Central to this process is the ATP-sensitive potassium (KATP) channel assembled from four pore-forming Kir6.2 subunits (encoded by KCNJ11) and four regulatory SUR1 subunits (encoded by ABCC8). KATP channels are gated by intracellular ATP and ADP, the concentrations of which change following glucose metabolism. This enables KATP channels to couple blood glucose levels with β-cell membrane potential to control insulin secretion. SUR1, a member of the ABC protein family, consists of a canonical ABC core structure of two 6-TM helix TM domains (TMD), TMD1 and TMD2, and two cytoplasmic nucleotide binding domains (NBDs), NBD1 and NBD2; in addition, it contains an N-terminal TM domain TMD0 which is connected to the ABC core via a cytoplasmic linker, L0.

To directly visualize how Aekatperone interacts with the channel we determined the cryoEM structure of KATP channels in the presence of 50 μM Aekatperone, using our published cryoEM sample preparation, imaging, and data processing workflow with specific modifications. 3D reconstruction of cryoEM particles of channels incubated with Aekatperone yielded a map with an overall resolution of 4.1 Å. A model built from the map shows a closed Kir6.2 channel pore with a pore radius of ~0.75 Å at the helical bundle crossing residue F168 and an inward-facing SUR1 with NBDs separated, resembling other inhibitor-bound KATP channel structures reported to date. A clear nonprotein density consistent with the size of Aekatperone (MW: 399.52 g/mol) was observed in a TM pocket above NBD1 in the ABC core of SUR1. Moreover, as in the structures of KATP bound to GBC, RPG, or CBZ, we observed clear cryoEM density corresponding to the Kir6.2 distal N-terminal peptide domain (KNtp) in between the two TM bundles of the SUR1-ABC core, with the very N-terminus of Kir6.2 contacting the bound Aekatperone. Stabilization of the KNtp-SUR1 interface promotes channel assembly, at the same time, it prevents Kir6.2 cytoplasmic domain from rotating to an open conformation, which explains the dual chaperone and inhibitor activity of Aekatperone. Aekatperone comprises a cyclohexane ring, a pyrazole, a sulfonamide moiety, a benzene ring, and an imidazole group. The preferred binding conformation, which accounted for the physical chemical properties of the compound and its surrounding interacting protein residues as well as fit to the cryoEM density, is shown in Figure 5B and C. In this structural model, the cyclohexyl moiety of Aekatperone is aligned with S1238 on the cytoplasmic end of the binding pocket, and the imidazole group is oriented toward the extracellular end of the binding pocket, interacting with the distal part of KNtp. The pyrazole moiety has its two nitrogen atoms coordinated by T1242 and N1245, while the sulfonyl moiety is oriented toward R1246 and R1300, each interacts with one of the two oxygens of the sulfonyl group.

>[4x]MLSRKGIIPEEYVLTRLAEDPTEPRYRTRERRARFVSKKGNCNVAHKNIREQGRFLQDVFTTLVDLKWPHTLLIFTMSFLCSWLLFAMVWWLIAFAHGDLAPGEGTNVPCVTSIHSFSSAFLFSIEVQVTIGFGGRMVTEECPLAILILIVQNIVGLMINAIMLGCIFMKTAQAHRRAETLIFSKHAVITLRHGRLCFMLRVGDLRKSMIISATIHMQVVRKTTSPEGEVVPLHQVDIPMENGVGGNSIFLVAPLIIYHVIDSNSPLYDLAPSDLHHHQDLEIIVILEGVVETTGITTQARTSYLADEILWGQRFVPIVAEEDGRYSVDYSKFGNTVKVPTPLCTARQLDEDRSLLDALTLASSRGPLRKRSVAVAKAKPKFSISPDSLS;> MPLAFCGTENHSAAYRVDQGVLNNGCFVDALNVVPHVFLLFITFPILFIGWGSQSSKVHIHHSTWLHFPGHNLRWILTFILLFVLVCEIAEGILSDGVTESRHLHLYMPAGMAFMAAITSVVYYHNIETSNFPKLLIALLIYWTLAFITKTIKFVKFYDHAIGFSQLRFCLTGLLVILYGMLLLVEVNVIRVRRYIFFKTPREVKPPEDLQDLGVRFLQPFVNLLSKGTYWWMNAFIKTAHKKPIDLRAIGKLPIAMRALTNYQRLCVAFDAQARKDTQSPQGARAIWRALCHAFGRRLILSSTFRILADLLGFAGPLCIFGIVDHLGKENHVFQPKTQFLGVYFVSSQEFLGNAYVLAVLLFLALLLQRTFLQASYYVAIETGINLRGAIQTKIYNKIMHLSTSNLSMGEMTAGQICNLVAIDTNQLMWFFFLCPNLWAMPVQIIVGVILLYYILGVSALIGAAVIILLAPVQYFVATKLSQAQRSTLEHSNERLKQTNEMLRGMKLLKLYAWESIFCSRVEVTRRKEMTSLRAFAVYTSISIFMNTAIPIAAVLITFVGHVSFFKESDLSPSVAFASLSLFHILVTPLFLLSSVVRSTVKALVSVKKLSEFLSSAEIREEQCAPREPAPQGQAGKYQAVPLKVVNRKRPAREEVRDLLGPLQRLAPSMDGDADNFCVQIIGGFFTWTPDGIPTLSNITIRIPRGQLTMIVGQVGCGKSSLLLATLGEMQKVSGAVFWNSNLPDSEGEDPSSPERETAAGSDIRSRGPVAYASQKPWLLNATVEENITFESPFNKQRYKMVIEACSLQPDIDILPHGDQTQIGERGINLSGGQRQRISVARALYQQTNVVFLDDPFSALDVHLSDHLMQAGILELLRDDKRTVVLVTHKLQYLPHADWIIAMKDGTIQREGTLKDFQRSECQLFEHWKTLMNRQDQELEKETVMERKASEPSQGLPRAMSSRDGLLLDEEEEEEEAAESEEDDNLSSVLHQRAKIPWRACTKYLSSAGILLLSLLVFSQLLKHMVLVAIDYWLAKWTDSALVLSPAARNCSLSQECDLDQSVYAMVFTLLCSLGIVLCLVTSVTVEWTGLKVAKRLHRSLLNRIILAPMRFFETTPLGSILNRFSSDCNTIDQHIPSTLECLSRSTLLCVSALTVISYVTPVFLVALLPLAVVCYFIQKYFRVASRDLQQLDDTTQLPLLSHFAETVEGLTTIRAFRYEARFQQKLLEYTDSNNIASLFLTAANRWLEVRMEYIGACVVLIAAATSISNSLHRELSAGLVGLGLTYALMVSNYLNWMVRNLADMEIQLGAVKRIHALLKTEAESYEGLLAPSLIPKNWPDQGKIQIQNLSVRYDSSLKPVLKHVNALISPGQKIGICGRTGSGKSSFSLAFFRMVDMFEGRIIIDGIDIAKLPLHTLRSRLSIILQDPVLFSGTIRFNLDPEKKCSDSTLWEALEIAQLKLVVKALPGGLDAIITEGGENFSQGQRQLFCLARAFVRKTSIFIMDEATASIDMATENILQKVVMTAFADRTVVTIAHRVHTILSADLVMVLKRGAILEFDKPETLLSQKDSVFASFVRADK> SDYVHEVPPPGEIVRPPIQLGETYYAVKNKAIASWVSIKVIEFTESTAINGNTMKSYKIRYLNTPYQMIKTVTAKHIAYFEPPPVRLTIGTRVIAYFDGTTLSRGKDKGVVQSAFYPGIIAEPLKQANRYRYLIFYDDGYTQYVPHRDVRLVCQASEKVWEDVHAASRDFIQKYVEKYSVDRPMVQCTRGQSM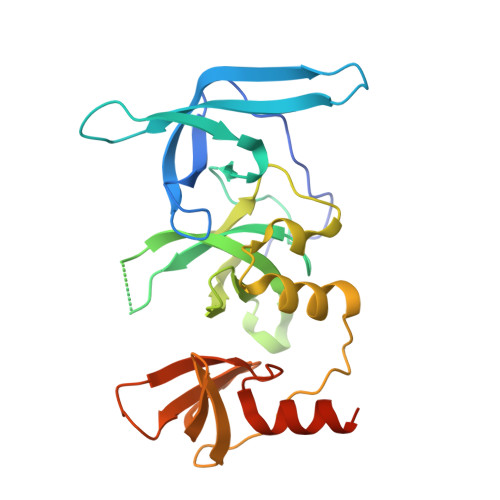TTESNGTWLYARVIDIDCSLVLMQFEGDKNHTEWIYRGSLRLGPVFRETQNNMNSSSAQQLRVP Lipins are magnesium-dependent phosphatidic acid phosphatases (PAPs) that catalyze the dephosphorylation of the membrane lipid phosphatidic acid (PA) to produce diacylglycerol (DAG). Our principal findings are that the M-Lip domain is a new protein fold that forms a dimer, binds membranes, and can affect lipin PAP activity, oligomerization, subcellular localization, and adipogenesis. Phospholipid synthesis and fat storage as triglycerides are regulated by lipin phosphatidic acid phosphatases (PAPs), whose enzymatic PAP function requires association with cellular membranes.

We, therefore, truncated the M-Lip domain of mouse lipin 1 to remove the C-terminal cluster of hydrophobic and basic residues implicated in membrane binding by HDX-MS. We refer to this construct as the M-Lipxtal domain. The M-Lipxtal domain could be purified without detergent and was extremely stable with a melting temperature of 65 °C. The structure of the M-Lipxtal domain of mouse lipin 1 was determined to resolutions of 1.5 Å and 1.9 Å in two unique space groups. Phases were obtained using single-wavelength anomalous diffraction from selenomethionine (SeMet)-derivatized protein. The structure of the M-Lipxtal domain revealed a protein fold with a three-stranded anti-parallel β-sheet at the core. Flanking the β-sheet were a set of two alpha helices (α1 and α2) and a short 3–10 helix (η1) that were oriented perpendicular to the β-sheet and two C-terminal α-helices (α3 and α4) that were oriented parallel to the β-sheet. Thus, the M-Lip domain represents a previously unrecognized and novel protein fold. Two additional peptides present in the crystallized M-Lipxtal domain were also protected. These peptides mapped to the same surface, which suggests that the core of the M-Lipxtal domain can also interact with membranes but is not the major determinant of membrane binding.

> SLRDLPSIAISLCGGLSDHREITKDAFLEQAVSYQQFADNPAIIDDPNLVVKVGNKYYNWTTAAPLLLAMQAFQKPLPKATVESIMRDKMP> GPLGSIAQARRQYHFESNQRTCNMTVLSMLPTLREALMQQLNSESLTALLKNRPSNK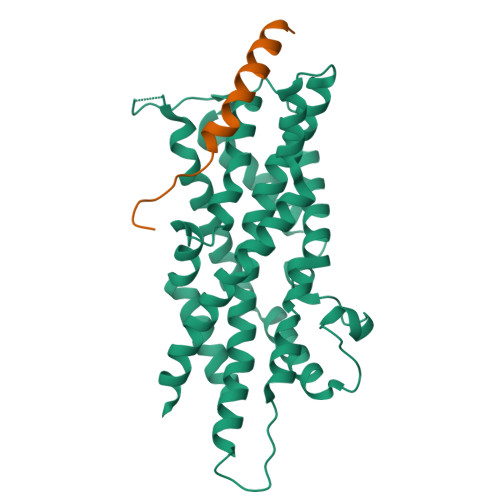LEIWEDLKIISFTRSTVAVYSTCMLVVLLRVQLNIIGGYIYLDNAAVGKNGTTILAPPDVQQQYLSSIQHLLGDGLTELITVIKQAVQKVLGSVSLKHSLSLLDLEQKLKEIRNLVEQHKSSSWINKDGSKPLLCHYMMPDEETPLAVQACGLSPRDITTIKLLNETRDMLESPDFSTVLNTCLNRGFSRLLDNMAEFFRPTEQDLQHGNSMNSLSSVSLPLAKIIPIVNGQIHSVCSETPSHFVQDLLTMEQVKDFAANVYEAFSTPQQLEK;> GPLGSMAAAEEGASVGAEADRELEELLESALDDFDKAKPSPAPPSTTTA>GFGNGNGFG[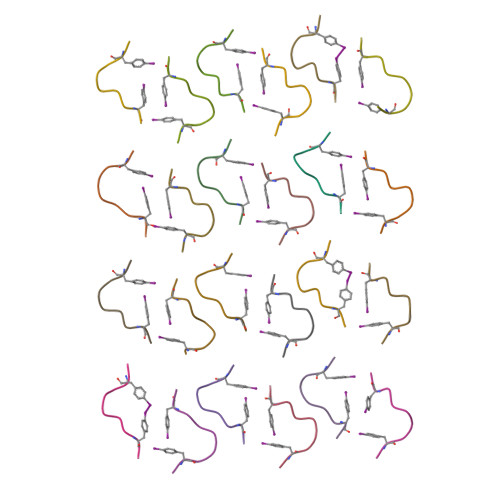24x]> SSSSESLSIIDVASDQNLFQTFIKEWRCKKRFSISLACEKIRGSGDDTLVVGLAVCWGGRDAYYFSLGGSGGLDPSLTLKDRMWYLQSCLRKESDKECSVVIYDFIQSYKILLLSCGISLEQSYEDPKVACWLLDPDSQEPTLHSIVTSFLPHELPLLEGMETSQGIQSLGLNAGSEHSGRYRASVESILIFNSMNQLNSLLQKENLQDVFRKVEMPSQYCLALLELNGIGFSTAECESQKHIMQAKLDAIETQAYQLAGHSFSFTSSDDIAEVLFLELKLPPGGSGGQFSTSKDVLNKLKALHPLPGLILEWRRITNAITKVVFPLQREKCLNPFLGMERIYPVSQSHTATGRITFTEPNIQNVPRDFEIKMGGSGGMPFSISMRHAFVPFPGGSILAADYSQLELRILAHLSHDRRLIQVLNTGADVFRSIAAEWKMIEPESVGDDDRQQAKQICYGIIYGMGAKSLGEQMGIKENDAACYIDSFKSRYTGINQFMTETVKNCKRDGFVQTILGRRRYLPGIKDNNPYRKAHAERQAINTIVQGSAADIVKIATVNIQKQLETFHSTFKSHGHREGMLQSDGGSGGCPIRGG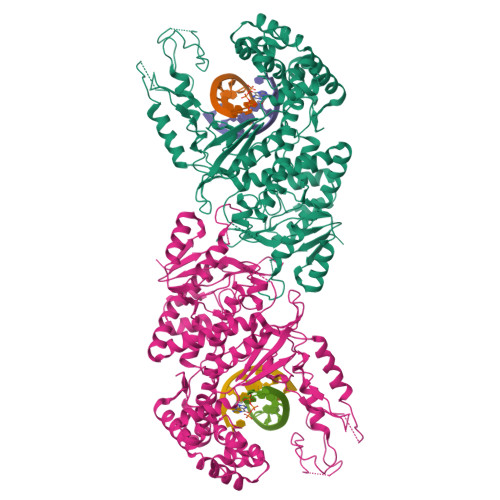FFILQLHDELLYEVAEEDVVQVAQIVKNEMESAVKLSVKLKVKVKIGASWGELKDFDV> MEHKAPLVEFLGLTFNLSDMLMITITCLIVFIIAVAATRSLQLRPTGMQNFMEWVFDFVRGIINSTMDWQTGGRFLTLGVTLIMYVFVANMLGLPFSVHVNGELWWKSPTADATVTLTLAVMVVALTHYYGVKMKGASDYLRDYTRPVAWLFPLKIIEEFANTLTLGLRLFGNIYAGEILLGLLASLGTHYGVLGAVGAAIPMMVWQAFSIFVGTIQAFIFTMLTMVYMAHKVSHDH;>EAAHGISGGTIIYQLLMFIILLALLRKFAWQPLMNIMKQREEHIANEIDQAEKRR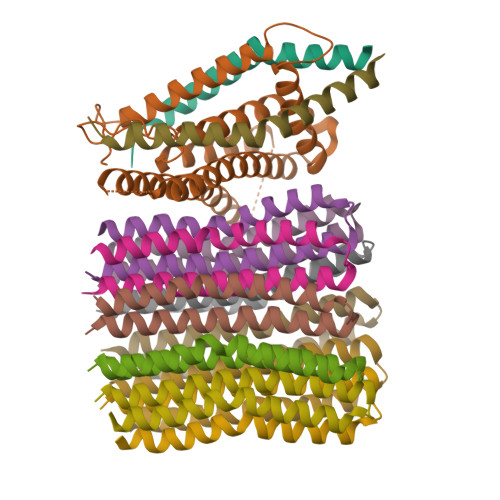QEAEKLLEEQRELMKQSRQEAQALIENARKLAEEQKEQIVASARAEAERVKETAKKEIEREKEQAMAALREQVASLSVLIASKVIEKELTEQDQRKLIEAYIKDVQEVGGAR[2x];>[10x]MSLGVLAAAIAVGLGALGAGIGNGLIVSRTIEGIARQPELRPVLQTTMFIGVALVEALPIIGVVFSFIYLGR> MNDRADFVVPDITTRKNVGLSHDANDFTLPQPLDRYSAEDHATWATLYQRQCKLLPGRACDE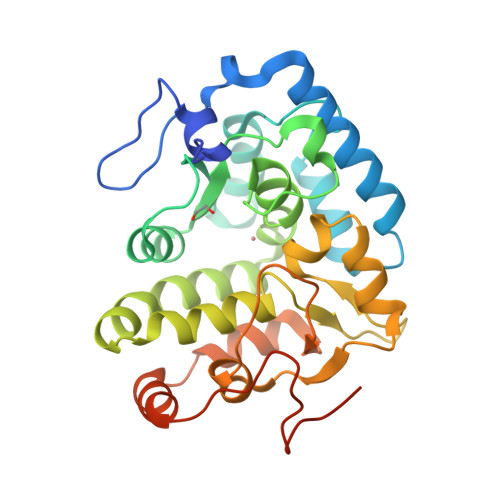FLEGLERLEVDADRVPDFNKLNEKLMAATGWKIVAVPGLIPDDVFFEHLANRRFPVTWWLREPHQLDYLQEPDVFHELFGHVPLLINPVFADYLEAYGKGGVKAKALGALPMLARLYWYTVEFGLINTPAGMRIYGAGILSSKSESIYCLDSASPNRVGFDLMRIMNTRYRIDTFQKTYFVIDSFKQLFDATAPDFAPLYLQLADAQPWGAGDIAPDDLVLNAGDRQGWADTEDV> MDMLSPVVREAEVSRAARRQSSNRKNPADESWSNATPTRGPSSRTTGQTLFRQHMTPQTWNSSRPPDVSAILGTVGRSPRLLQTPGRLANLSMMSNPDDSVWTTTFSPGRTGMYTTLDSPSFTEDITLSAVMLQEEDPGEAATMSMYPDFLKSFLEHPSSAVFELIEQYEATCNTQITLLKKIVKRVTPGQQKFSKTASILWLLQQEMVTWRLIAALYRDRIQSALEEENMFEIAAPNASEKTIVDKLFQRDTLVRQSQLVVDWLESIAKDEVGDFSDNIEYYAKSVYWENTLHTLKQRSMLSLGSSRPLVSELDPDAPIRQKLPLDDLDREDDIRLLKYLFTLIRAGMTDEAQRLCKRCGQAWRAATLEGWKLYHDANINGGTELQAVEGNPYRCVWKTCCWRMAEDEQFNKYERAIYATLSGNLKQLLPVCESWEDTVWAHFKVMVDSLVEQEIRASIISFNEANELPREYLEANWTLDSVFEELQATDKKRVLEENREHYHIIQKFVILADVDGLMDEFSEWLSNGKNLLLGHLLRFMTHLLLFFRTLGLQAKEEVSVEVLKTYIQRLINEK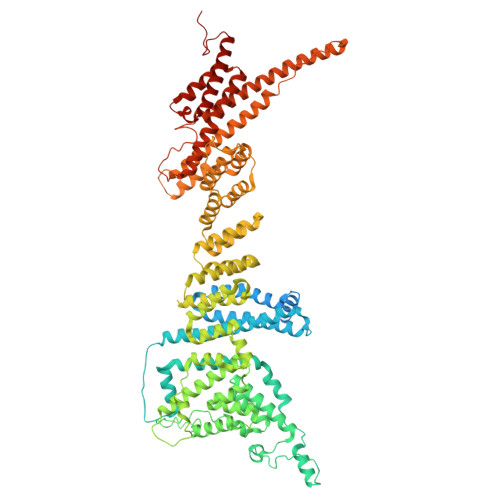QIELIAFYVSHLPQELAISQYAVFLENITDPDQRQRCLELAKEAGLDVASITKTVVENTRKKDAGEFAHHDFAPALDSGTSEEDRAKIDVIDWLVFDPAQRAEALKQSNAIMRKFLASKKHEAAKEVFAKIPQDSIAEIYSQWEEQAMDSALPAEDDNAIREHLCIRAYLESHEAFNEWFKHINSPPQKPTLVGQASFTEKVAHEHKEKKYEMDFGIWKGHLDALTSDVKEKIYNVLLFVDGGWMVDVREDTEEDPERSHQMVLLRRLCLPMMCFLLHTVLHNTKQYKDCLRLADIVSSENQKLYTVFSKTEMRNLLQKLRESSLMLLDLQLDPLGYEIQS>SNKVGTLQAQVEATQKQKAQPIDANRKYDYKLQYYLNDYVYAYFTLPQEGDKQQAQVEHLNSFYNFVPDVKAQGQVRNPSTLLDSQLVTVEGKVATYKVKYKEMIQHDKDTEEKELVTGFNIPFDEKEGKYYVSGLPWFSCIESSQAGYFSEDDQLQLTANDHVSDSQHKKVEKFLKVFFTNYTTNQDNLNLIA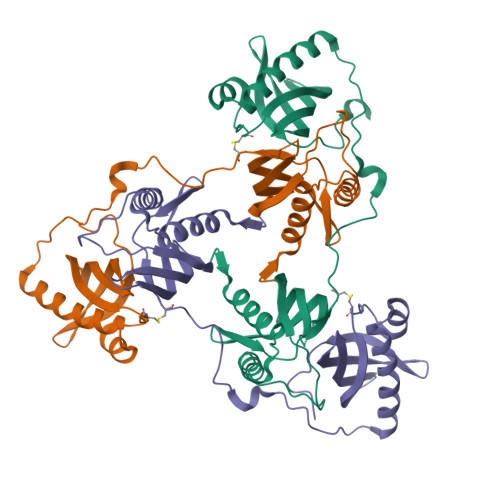KNVAIVCNTTFKTIDYTYLKKDRADLIAYVQATFEVGGTTHSENFTFTLSEKDKSYYVTKLEHTIPLNYANDKD[3x]>[2x]MADKELKFLVVDDFSTMRRIVRNLLKELGFNNVEEAEDGVDALNKLQAGGYGFVISDWNMPNMDGLELLKTIR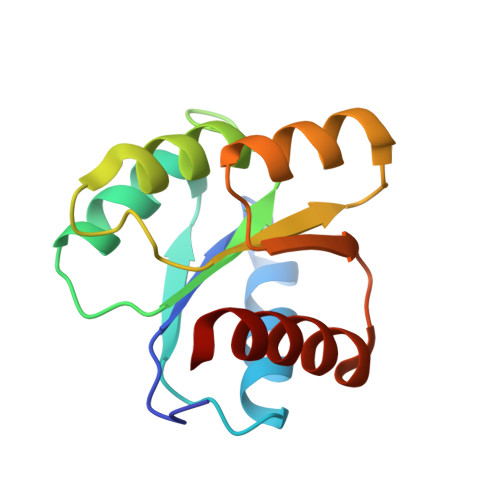ADGAMSALPVLMVTAEAKKENIIAAAQAGASGYVVKPFTPATLEEKLNKIFEKLGM4-chlorophenol | C6 H5 Cl O 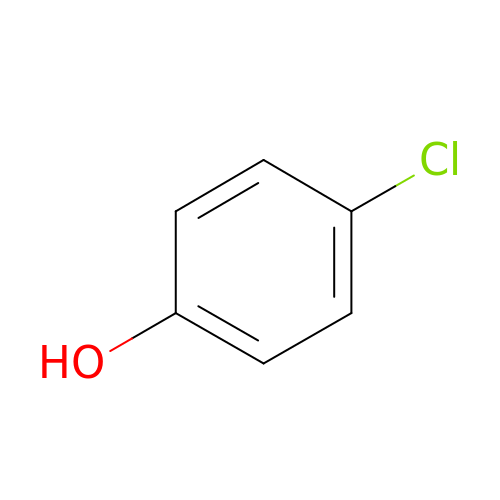| WXNZTHHGJRFXKQ-UHFFFAOYSA-N>[2x]AGIHHHHHHSSEPSCRFAHQYTQEQVLQNPSKFINDVLFWEGKFHQNNISYNSGNGMSYDGTNIDWVTGEGTVKHPFSAASKESLQVMLYAHAIAGSADAARFLSPNNPSAAPGIAASIMDTKLQTYLRFNET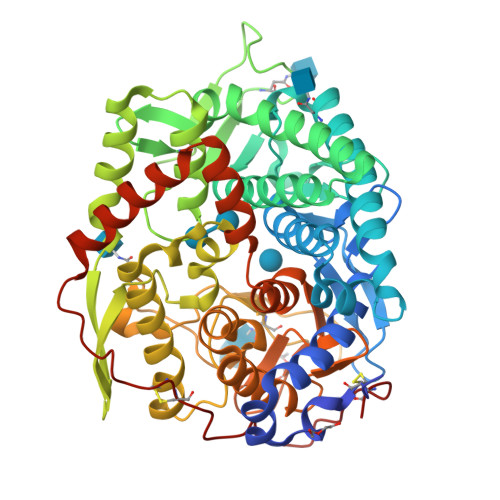YPGFGGFLPWFTSSSQDLTPTWDWNNRVPGLDNGELLWAVYAFIQAAENTSNKSFIDLAKKWQTWMDYTKTTAAHIFYQGEGKVCAVTDIKNQSLPVYHPEQTYACEGTSYLNDPYEGELFTWWLQFFGGLSDADIEALWEYKRPQLVSVDYHIGNVGPITVQKGYWFSSHETWKVLEMPYYDIDIIRRVFQNAERARTCNSVVTQVPGMFASINNVTDPATGDVVGYISNAGIPSIANQTIQELDVITPYSVFPTVLFDKGVGMAWWRNMAIGKKMQNIYGSTESTRRDGTGVSALLTWDSKVSTVNAILGGVSGLVSQKMKAENIYNTFVERIEAEYSRVFKNLKGEHVPFCLPQETVPDTGLVDFTTCN> SSQIRQNYSTEVEAAVNRLVNLYLRASYTYLSLGFYFHRDDVALEGVCHFFRELAEEKREGAERLLKMQNQRGGRALFQDLQKPSQDEWGTTLDAMKAAIVLEKSLNQALLDLHALGSAQADPHLCDFLESHFLDE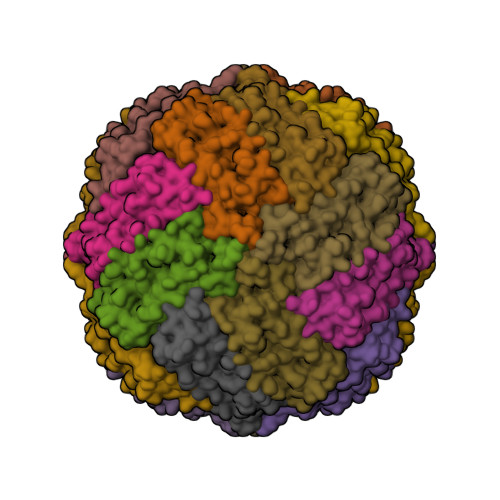EVKLIKKMGDHLTNIQRLVGSQAGLGEYLFERLTLKHD Acylpeptide hydrolase (APEH) or acylaminoacyl‐peptidase (AAP) is a serine hydrolase that regulates protein metabolism. It can also bind to and process unusual substrates, acting as a detoxifier. The most prominent physiological function of APEH is the removal of N‐acetylated amino acids from the N‐terminus of oligopeptides and proteins (Perrier et al., 2005) thereby exerting crucial control over the proteasomal degradation of damaged and misfolded proteins (Adibekian et al., 2011; Hoernstein et al., 2023; Hwang et al., 2010; Palmieri et al., 2011; Sandomenico et al., 2021; Shimizu et al., 2003; Shimizu et al., 2004; Tangri et al., 2021). The S9 serine protease subfamily, the so‐called oligopeptidases, employs a further, size‐based selection process (Kobayashi & Smith, 1987). Their active site is sequestered in an inner pocket that is formed between the catalytic hydrolase domain and a propeller domain that caps it.

To further probe the catalytic significance of the shift of the oxyanion loop, we produced PhAPEH and ApAPEH. Not only is the shape and position of the oxyanion loop unchanged by complex formation in these archaeal variants, but it is also locked in a conformation that is very similar to its forward shifted state in pAPEH; thus, these systems can be used as functional models of the enzyme with a more restricted and confined catalytic site. We found that the archaeal variants are quite selective toward their specific substrate Ac‐Leu‐pNA, not being able to cleave Ac‐Ala‐pNA, while pAPEH processes both almost instantaneously. Furthermore, neither ApAPEH nor PhAPEH is inhibited by meropenem, the bulky carbapenem antibiotic that is a potent inhibitor of pAPEH (Kiss‐Szemán, Stráner, et al., 2022). Attempts at producing a co‐crystal structure of ApAPEH and meropenem were also unsuccessful—using the same protocol that afforded co‐crystals of ApAPEH with peptide‐like chloromethyl ketone inhibitor (Menyhárd et al., 2015; see Data S1, Chapter II: “Substrate/inhibitor preference of APEH from Aeropyrum pernix and Pyrococcus horikoshii”). Conversely, it seems that archaeal variants of APEH contain a pre‐formed reactive center that requires no adjustment upon ligand binding. However, no such shift is caused by the binding of CMK‐derivatives by the archaeal variants of the enzyme. In fact, both the size and the invariability of the active site of ApAPEH (or ApAAP) and PhAPEH (or PhAAP) are closer to those of the “regular” serine hydrolases than to those of pAPEH. Here, we established that this same Pro is also the most likely inducer of the backward shift and flexibility of the oxyanion‐loop, and also demonstrated that archaeal variants that carry Val at this position do not show the same promiscuity (Chapter II: Substrate/inhibitor preference of APEH from Aeropyrum pernix and Pyrococcus horikoshii).

>MRIIMPVEFSRIVRDVERLIAVEKYSLQGVVDGDKLLVVGFSEGSVNAYLYDGGETVKLNREPINSVLDPHYGVGRVILVRDVSKGAEQHALFKVNTSRPGEEQRLEAVKPMRILSGVDTGEAVVFTGATEDRVALYALDGGGLRELARLPGFGFVSDIRGDLIAGLGFFGGGRVSLFTSNLSSGGLRVFDSGEGSFSSASISPGMKVTAGLETAREARLVTVDPRDGSVEDLELPSKDFSSYRPTAITWLGYLPDGRLAVVARREGRSAVFIDGERVEAPQGNHGRVVLWRGKLVTSHTSLSTPPRIVSLPSGEPLLEGGLPEDLRRSIAGSRLVWVESFDGSRVPTYVLESGRAPTPGPTVVLVHGGPFAEDSDSWDTFAASLAAAGFHVVMPNYRGSTGYGEEWRLKIIGDPCGGELEDVSAAARWARESGLASELYIMGYSYGGYMTLCALTMKPGLFKAGVAGASVVDWEEMYELSDAAFRNFIEQLTGGSREIMRSRSPINHVDRIKEPLALIHPQNASRTPLKPLLRLMGELLARGKTFEAHIIPDAGHAINTMEDAVKILLPAVFFLATQRERR[4x]>[4x]GPTPEAPYASLTEIEHLVQSVCKSYRETCQLRLEDLLRQRSNIFSREEVTGYQRKSMWEMWERCAHHLTEAIQYVVEFAKRLSGFMELCQNDQIVLLKAGAMEVVLVRMCRAYNADNRTVFFEGKYGGMELFRALGCSELISSIFDFSHSLSALHFSEDEIALYTALVLINAHRPGLQEKRKVEQLQYNLELAFHHHLCKTHRQSILAKLPPKGKLRSLCSQHVERLQIFQHLHPIVVQAAFPPLYKELFSTTETESPVGLSK;>[4x]EFPYLLSLLGEVSPQ

Retinoid-related orphan receptor gamma (RORγ) is a transcription factor belonging to a sub-family of nuclear receptors that includes two closely related members RORα and RORβ. The nuclear hormone receptor RORγ regulates transcriptional genes involved in the production of the pro-inflammatory interleukin IL-17 which has been linked to autoimmune diseases such as rheumatoid arthritis, multiple sclerosis and inflammatory bowel disease. This transcriptional activity of RORγ is modulated through a protein-protein interaction involving the activation function 2 (AF2) helix on the ligand binding domain of RORγ and a conserved LXXLL helix motif on coactivator proteins. The conformation of the AF2 helix can be modulated through targeted ligands which bind the LBS and increase the binding of the coactivator protein (agonists) or disrupt binding (inverse agonists) thereby enhancing or inhibiting transcription.

Using a FRET based assay we discovered agonist BIO592 which increased the coactivator peptide TRAP220 recruitment to RORγ (EC50 0f 58nM and Emax of 130 %) and a potent inverse agonist BIO399 which inhibited coactivator recruitment (IC50: 4.7nM). RORγ518 bound to agonist BIO592 was crystallized with a truncated form of the coactivator peptide EBI96 to a resolution of 2.6 Å. The structure of the ternary complex had features similar to other ROR agonist coactivator structures in a transcriptionally active canonical three layer helix fold with the AF2 helix in the agonist conformation. The agonist conformation is stabilized by a hydrogen bond between His479 and Tyr502, in addition to π-π interactions between His479, Tyr502 and Phe506. The hydrogen bond between His479 and Tyr502 has been reported to be critical for RORγ agonist activity. Electron density for the coactivator peptide EBI96 was observed for residues EFPYLLSLLG which formed a α-helix stabilized through hydrophobic interactions with the coactivator binding pocket on RORγ. BIO592 bound in a collapsed conformational state in the LBS of RORγ with the xylene ring positioned at the bottom of the pocket making hydrophobic interactions with Val376, Phe378, Phe388 and Phe401, with the ethyl-benzoxazinone ring making several hydrophobic interactions with Trp317, Leu324, Met358, Leu391, Ile 400 and His479. The sulfonyl group faces the entrance of the pocket, while the CF3 makes a hydrophobic contact with Ala327.>MNHKVHHHHHHIEGRHMGTTPSDPPTNPP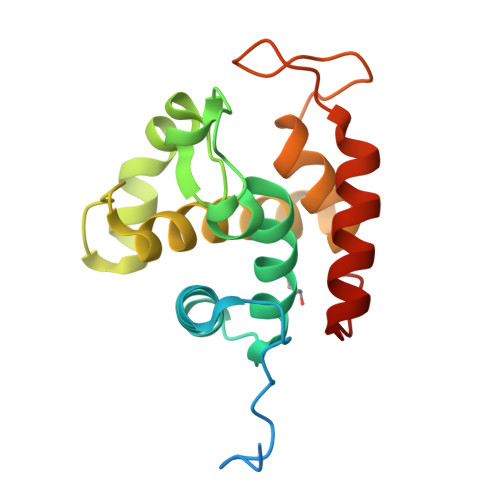TTVTKPAEVPSRIWTYVMNADNAYGKGGDFALLLSAVIKKESYFGDGLSGSPSAGDGLMQVEPNTRNAYLSQFSAKYGHAYNHSSEQDQVYMGSLILNEKIVRFGSIYSGLLHYNGGDYWYPGATDSYGRPILADQYANTVYAQYKSYGGRYSR[4x]> GSTTPLLANSLSVHQLAAQGEMLYLATRIEQENVINHTDEEGFTPLMWAAAHGQIAVVEFLLQNGADPQLLGKGRESALSLACSKGYTDIVKMLLDCG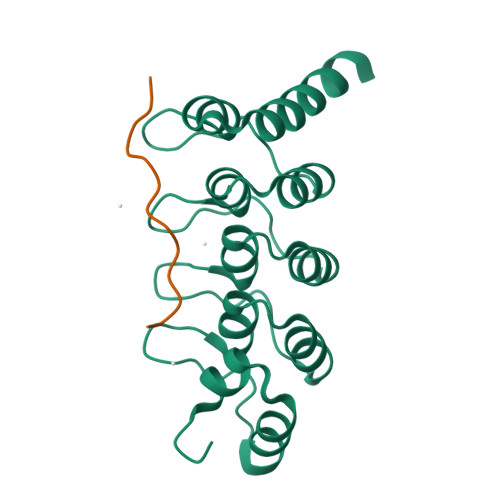VDVNEYDWNGGTPLLYAVHGNHVKCVKMLLESGADPTIETDSGYNSMDLAVALGYRSVQQVIESHLLKLLQNIKE;> RAFWHTPRLPTLPKRVP> GSHMASEKGTVVTETADDDLFTTYRLDLEDARSKEREELNAIVSSDDAT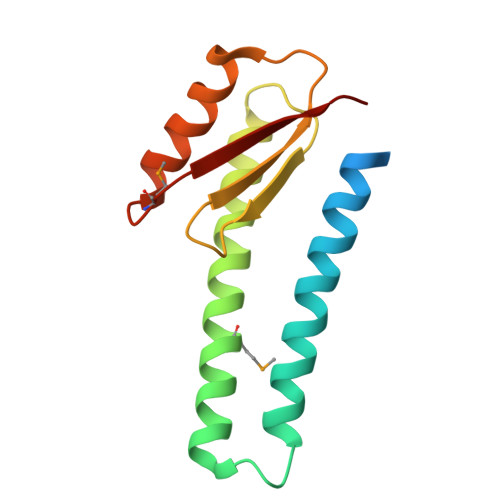AKEKSEAYDKMTALSEVEGTEKQLETLIKTQGYEDALVNAEGDKINITVKSDKHSKSKATAIIDLVAKEIKTMKDVAVTFEPSK In plant cells, ALMTs are key plasma and vacuolar membrane-localized anion channels regulating plant responses to the environment. Among the different ion transporters and ion channels localized in the vacuolar membrane, the ion channels of the aluminum-activated malate transporter (ALMT) family play a key role for the transport of chloride and malate during stomata opening/closure. ALMTs are also involved in transporting various anion including chloride, nitrate, fumarate, tartrate, citrate, and malate. Here we report the cryo-EM structures of ALMT9 from Arabidopsis thaliana (AtALMT9), a malate-activated vacuolar anion channel, in plugged and unplugged lipid-bound states.

AtALMT1 shows aluminum-induced activation within minutes and mediates voltage-dependent malate efflux conferring aluminum tolerance. Addition of a detergent LMNG may have introduced artifacts in protein purification. Notably, the purification of GmALMT12/QUAC1 whose structure has fenestration employed LMNG for purification. To check whether lateral fenestrations are artifacts from our purification protocol, we determined the cryo-EM structure of AtALMT1 with the same purification method as with our AtALMT9. AtALMT1 of the clade 1 possesses no fenestration, and the conserved threonine residues apparently stabilize the selectivity filter. T61 directly interacts with R80; T84, T144, and W57 (W120 of AtALMT9) make a hydrophilic pocket for positioning of R165.

>[2x]MEKVREIVREGIRVGNEDPRRIIHAFKVGLALVLVSSFYYYQPFGPFTDYFGINAMWAVMTVVVVFEFSVGATLGKGLNRGVATLVAGGLGIGAHQLARLSGATVEPILLVMLVFVQAALSTFVRFFPWVKTKFDYGILIFILTFALISLSGFRDEEIMDLAESRLSTVVIGGVSCILISIFVCPVWAGQDLHSLLASNFDTLSHFLQDFGDEYFEAREKGDYKVVEKRKKNLERYKSVLDSKSDEEALANYAEWEPPHGQFRFRHPWKQYVAVGALLRQCAYRIDALNSYINSDFQIPVDIKKKLETPLRRMSSESGNSMKEMSISLKQMIKSSSSDIHVSNSQAACKSLSTLLKSGILNDVEPLQMISLMTTVSMLIDIVNLTEKISESVHELASAARFKNKMRPTVLYEKSDSGSIGRAMPIDSHEDHHVVTVLHDVDNDRSNNVDDSRGGSSQDSCHHVAIKIVDDNSNHEKHEDGEIHVHTLSNGHLQ> 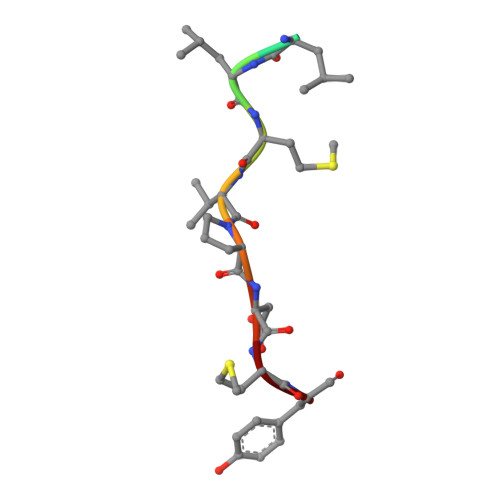XELLMVPDMY6-chloro-N-[(furan-2-yl)methyl]pyrazin-2-amine 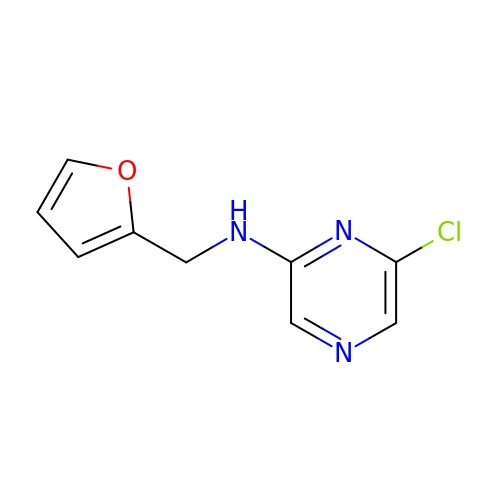| C9 H8 Cl N3 O | PEEZSSNXCUTRPK-UHFFFAOYSA-N>ETGKPTCDEKYANITVDYLYNKETKLFTAKLNVNENVECGNNTCTNNEVHNLTECKNASVSISHNSCTAPDKTLILDVPPGVEKFQLHDCTQVEKADTTICLKWKNIETFTCDTQNITYRFQCGNMIFDNKEIKLENLEPEHEYKCDSEILYNNHKFTNASKIIKTDFGSPGEPQIIFCRSEAAHQGVITWNPPQRSFHNFTLCYIKETEKDCLNLDKNLIKYDLQNLKPYTKYVLSLHAYIIAKVQRNGSAAMCHFTTKSAPPSQVWNMTVSMTSDNSMHVKCRPPRDRNGPHER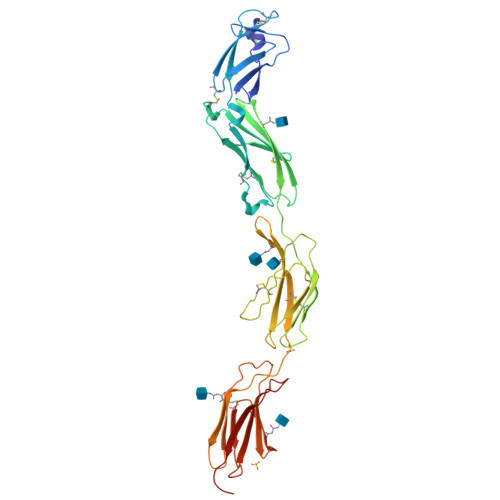YHLEVEAGNTLVRNESHKNCDFRVKDLQYSTDYTFKAYFHNGDYPGEPFILHHSTSGTKHHHHHH[2x]> ASTPVFWDDPQNHTFRHTLFCQDGIPNIGLSETYDEDELFSFDFSQNTRVPRLPDFAEWAQGQGDASAIAFDKSFCEMLMREVSPKLEGQIPVSRGLPVAEVFTLKPLEFGKPNTLVCFISNLFPPTLTVNWQLHSAPVEGASPTSISAVDGLTFQAFSYLNFTPEPFDLYSCTVTHEIDRYTAIAYWVPQ;> GFVAHVESTCVLNDAGTPQDFTYCVSFNKDLLACWDPDVGKIVPCEFGVLSRLAEIISNILNEQESLIHRLQNGLQDCATHTQPFWDVLTHRTRAPSVRVAQTTPFNTREPVMLACYVWGFYPADVTITWMKNGQLVPSHSNKEKTAQPNGDWTYQTVSYLALTPS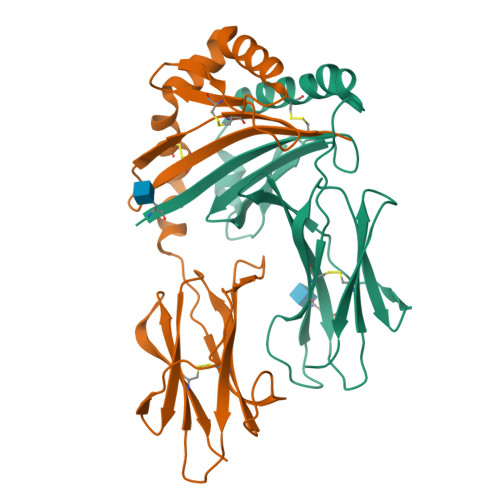YGDVYTCVVQHSGTSEPIRGDWTPG>[2x]MASMTGGQQMGAPITAYAQQTRGLLGCIITSLTGR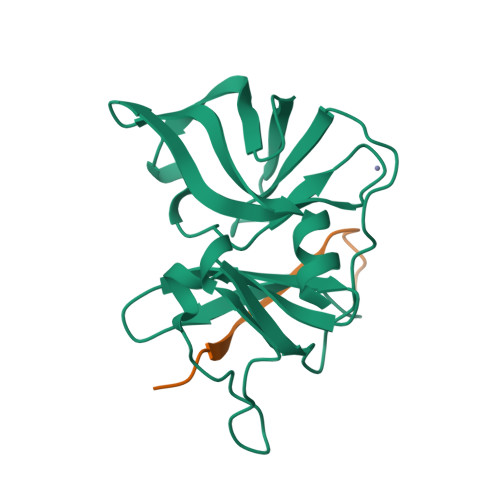DKNQVEGEVQIVSTATQTFLATCINGVCWTVYHGAGTRTIASPKGPVIQMYTNVDQDLVGWPAPQGSRSLTPCTCGSSDLYLVTRHADVIPVRRRGDSRGSLLSPRPISYLKGSSGGPLLCPAGHAVGLFKAAVCTRGVAKAVDFIPVENLETTMRSGSHHHHHH;>[2x]KGSVVIVGRIVLSGKPAIIPA> MKKAVINGEQIRSISDLHQTLKKELALPEFYGENLDALWDCLTGWVEYPLVLEWRQFEQS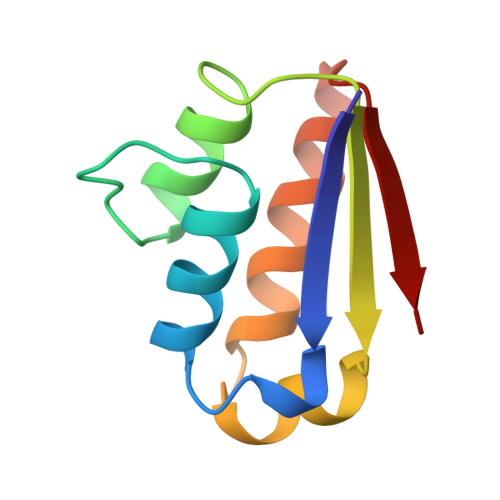KQLTENGAESVLQVFREAKAEGCDITIILS>MQDVRVQVLPEVRGQLGGTVELPCHLLPPVPGLYISLVT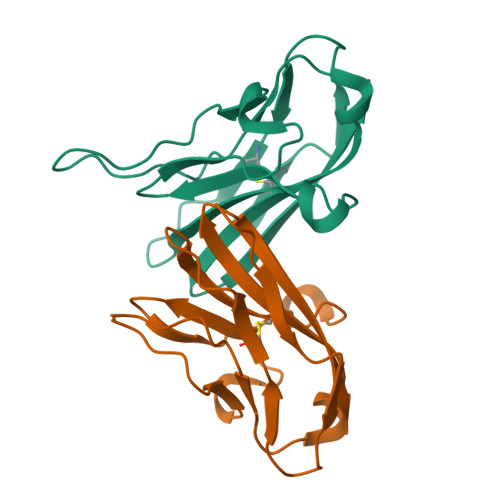WQRPDAPANHQNVAAFHPKMGPSFPSPKPGSERLSFVSAKQSTGQDTEAELQDATLALHGLTVEDEGNYTCEFATFPKGSVRGMTWLRV[2x]>HMLDEPPEGFPEPLNPTNFKEELSKGLHIIDFYSPYCPHCKHLAPVWM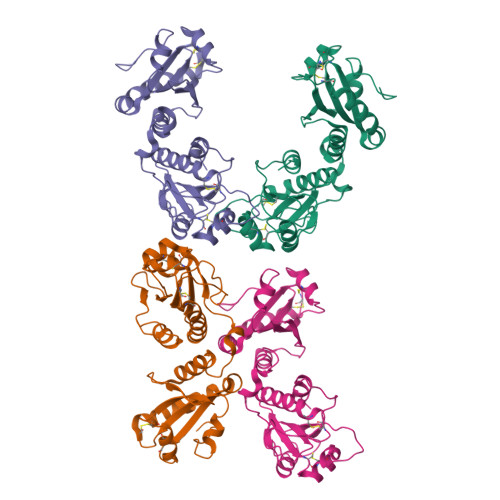ETWEEFKEESKTLNITFSQVNCIESADLCGDENIEYFPEIRLYNPSGYIKSFTETPRTKESLIAFARRESMDPNNLDTDLDSAKSESQYLEGFDFLELIAGKATRPHLVSFWPTKDMKNSDDSLEFKNCDKCHEFQRTWKIISRQLAVDDINTGHVNCESNPTICEELGFGDLVKITNHRADREPKVALVLPNKTSNNLFDYPNGYSAKSDGYVDFARRTFTNS[4x]> GSAQADFDIPAGPLAPALAHFGQSAHILLSYPTALTEGRSTSGLAGRFDIDQGLAILLAGTGLEASRGANASYSLQASASTG;> GAMGQDWRADYHSRIGEQRRLTLADGTQVQLNTDSALNVAFDQQARRLRLVRGEMLITRPALADSRPLWVDTEHGRLESTLAQFNVRLHGQHTQATVYQGSVALQPALHAYPPILLGAGEQASFNQQGLLARQAVAAVAPAWSQGMLVAQGQP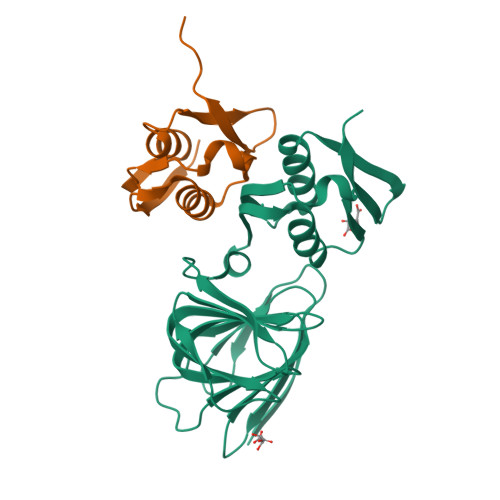LAAFIEDLARYRRGHLACDPALAGLRVSGTFPLENTDKIIAAVAETLQLEVQHFTRYWVTLKPRMA> GMEADARSIYVGNVDYGATAEE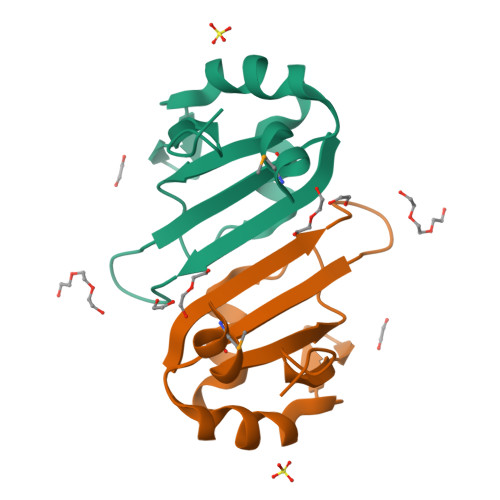LEAHFHGCGSVNRVTILCDKFSGHPKGFAYIEFSDKESVRTSLALDESLFRGRQIKVIPKRTNRPGI>MRTLLIMAVLLLGVEGS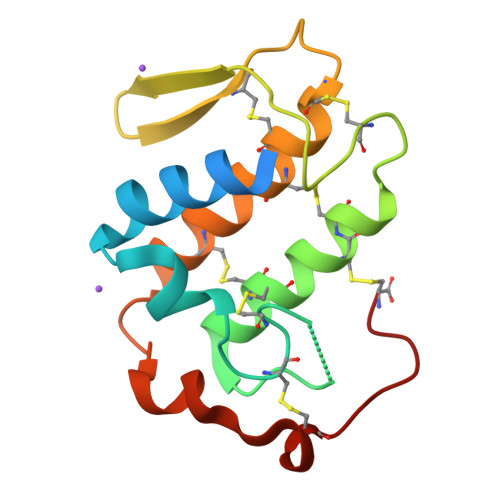LLQLRKMIKKMTNKEPILSYSKYGCNCGMAGRGKPVDATDTCCSIHNCCYGKVTSCSTKWDSYSYSWENGDIVCDEKHPCKDVCECDKAVATCFRDNLDTYKKRNIFHPTSSCVKVSTPC[3x]>[4x]MTIFQFPQDFMWGTATAAYQIEGAYQEDGRGLSIWD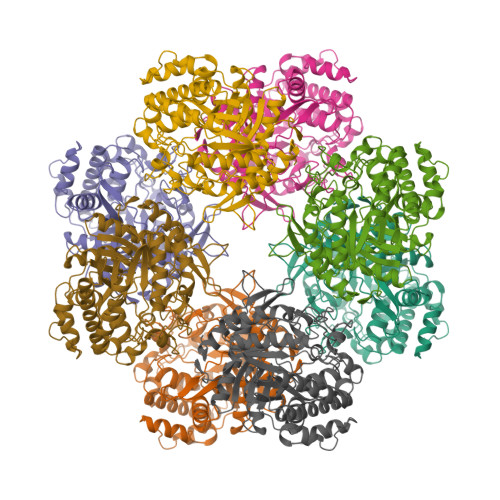TFAHTPGKVFNGDNGNVACDSYHRYEEDIRLMKELGIRTYRFSVSWPRIFPNGDGEVNQEGLDYYHRVVDLLNDNGIEPFCTLYHWDLPQALQDAGGWGNRRTIQAFVQFAETMFREFHGKIQHWLTFNEPWCIAFLSNMLGVHAPGLTNLQTAIDVGHHLLVAHGLSVRRFRELGTSGQIGIAPNVSWAVPYSTSEEDKAACARTISLHSDWFLQPIYQGSYPQFLVDWFAEQGATVPIQDGDMDIIGEPIDMIGINYYSMSVNRFNPEAGFLQSEEINMGLPVTDIGWPVESRGLYEVLHYLQKYGNIDIYITENGACINDEVVNGKVQDDRRISYMQQHLVQVHRTIHDGLHVKGYMAWSLLDNFEWAEGYNMRFGMIHVDFRTQVRTPKESYYWYRNVVSNNWLETRR> GAMGIRNSKAYVEHRLRAAEHPRPDYVLLHISDTHLIGGDRRLYGAVDADDRLGELLEQLNQSGLRPDAIVFTGDLADKGEPAAYRKL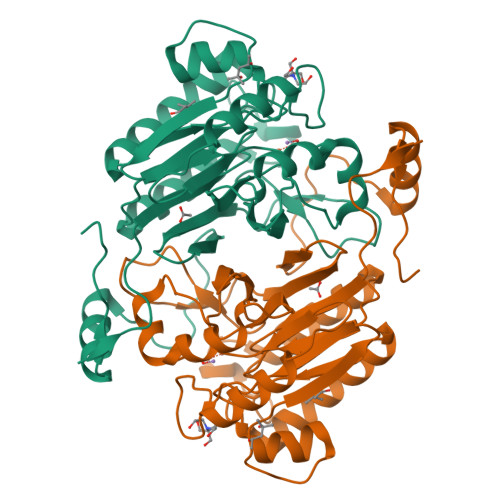RGLVEPFAAQLGAELVWVMGNHDDRAELRKFLLDEAPSMAPLDRVCMIDGLRIIVLDTSVPGHHHGEIRASQLGWLAEELATPAPDGTILALHHPPIPSVLDMAVTVELRDQAALGRVLRGTDVRAILAGHLHYSTNATFVGIPVSVASATCYTQDLTVAAGGTRGRDGAQGCNLVHVYPDTVVHSVIPLGGGETVGTFVSPGQARRKIAESGIFIEPSRRDSLFKHPPMVLTSSAPRSPVD>[2x]SFDKTTFRLLRGESNLFYTLAKWENNKLHVELPENIDKQSPTMTLIYDENGQLLWAQRDVPWLMKMIQPDWLKSNGFHEIEADVNDTSLLLS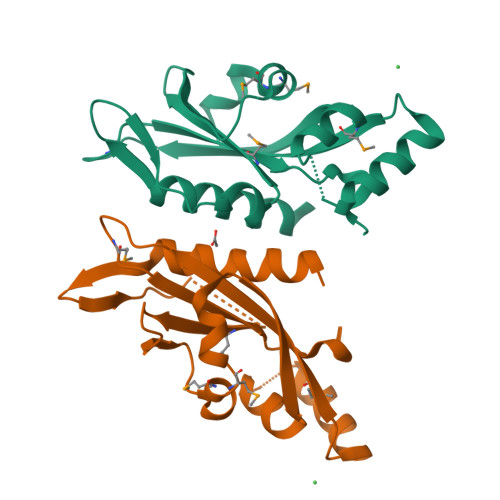GDHSIQQQLQEVREDDDDAEMTHSVAVNVYPATSRMPKLTIVVVDTIPVELKSSYM> SNAQIIFNVHPAPTRKIAVAKQNYRCAGCGIRTDPDYIKRLRYCE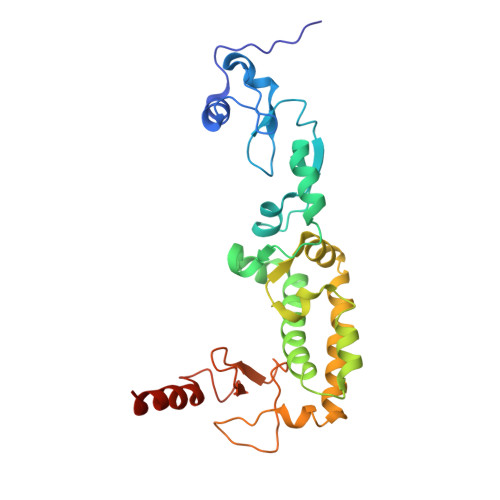YLGKYFCQCCHENAQMAIPSRVLRKWDFSKYYVSNFSKDLLIKIWNDPLFNVQDINSALYRKVKLLNQVRLLRVQLCHMKNMFKTCRLAKELLDSFDTVPGHLTEDLHLYSLNDLTATRKGELGPRLAELTRAGATHVERCMLCQAKGFICEFCQNEDDIIFPFELHKCRTCEECKACYHKACFKSGSCPRCERLQARREALARQSLES> MDKEIYCGSVPVSYFDPFDLFESLRPEFQQILPLDNIHWKAFDGTVRTVNRLPIELIPEGRGEADKSNDEQPFIRFLIVNCISIDQYRAKVRPLVRQWLPNLESVSSSTGEKMIYKPIILLYANSEVVDSNLFKSVSLMEKFGKDFPHVQTLEVRSVYRSPKERQEFWNQFSQKIKASVLSIFQKRLTHLQHSLANLQKGNNFEEQLLTREKLYELYVVFNILEDASLELQKIKKEILRRNMNMPDGKLQVPFESSSKSDESLGSIIIEGTLDKFQLHKYFFIRRLRLLKLEDQTLTAFVGAFQLIKNFIESISIEYRKSVRLLEFKHYFITSMLSYFEFENVSNPLLCEIKAELLMLKRDNWVQ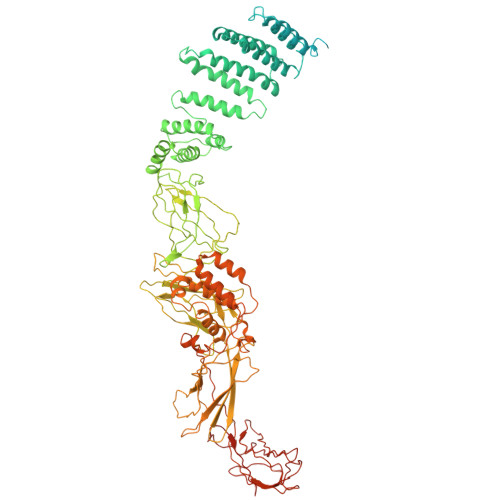GVMATSGYRLMDKNYPNSDVKYKFDLLKETFVDETVFQENFLTLTKEILSLFNKCEGKRQRIVDILSIEIGLLYYQGKKYEEAVSLFLSCYEYYTQTNKNSIGLKILQVFIDSLSHCPKLDVLQIDGESVSASAVLTNAFLNILKLCKDNDSKEIWWKKFMDLQMKNNIHLMYPLDGLFEVTLNSKVHLARANVSAIEVNLKSYGFPEDISTKTMRLSLKNMGGDVIVFGASDFLLKKGENKLILECRDIMYGEFSLLSFEIIVEGITFVKEFPENQDEFIVVPEIYCKESTKVLVKQAHNLNLGEYALELKSVQSDALESLQVEVEVQKNIGNMKNLPVSFSMDEIQARKRYNTPFENVRLEYYLLDQITAFDLIIKTSFTKKNDQGTFGETKKVRIQCYLQLSVSVEDIFKKDIFFFKFLLNSSVREEPVILYSSELSAPDTRNDYNIRGDYIATTPALITFDGNESFINCYEITANNNFDSKDIFNLKVRYNTLKEQLDCFITDAVLIEGDVEWFILFEKWKTFWELEILKKLKYDYDAFKENRIIRLLKTSIDLNKTKSKIRNLCIEKAVLDKILICLNKVSRGIAVCNTDMDEYVRNLVPKQLTVPVQLPGFEQFFHVQFEQMETSHDALHDTIATIGNSLSYTVIVENLSGQWGQDVIDDGGYIFEILSSNEWLIHGQKRCAIKEKRKEFEVHLIPLKKGYLNFPRVEITNINGKSCRVDHSNAFESILIF>[2x]MLRSTHSPSGSSSAAPASSSSDAAMVGGGGAAAAAGSGGAPSGAKLLQILNVRVVGNGDRVVVLSHGFGTDQSAWSRVLPYLTRDHRVVLYDLVCAGSVNPEHFDFRRYDTLDSYVDDLLAILDALRIPRCAFVGHSVSAMIGILASIRRPELFAKLVLIGASPRFLNDNDYHGGFELPEIQQVFDAMAANYSAWAVGYAPLAVGADVPAAVQEFSRTLFNMRPDISLHVCRTVFNTDLRGVLGMVRSPCVVVQTTRDVSVPASVAAYLRAHLGGRTTVEFLQTEGHLPHLSAPGLLAQVLRRALARY

Strigolactones (SLs) are a class of important plant hormones mainly regulating plant architecture such as branching, which is crucial for crop yield. Different from other receptors, which could only sense hormone molecules, the receptor D14 have dual roles to sense and hydrolyze SL, demonstrating a brand-new function mode. During the hydrolysis of SL, D14 covalently binds to the D-ring at the catalytic center, then it associates with downstream protein MAX2/D3 to form D14–MAX2/D3 SCF E3 complex. This ubiquitin ligase complex will recruit the downstream transcription repressors SMXL6/7/8/D53, leading to the degradation of SMXLs/D53 through the 26S proteasome pathway.

Here, two putative SL receptors SsD14a/b and the interacting F-box protein SsMAX2 were identified in Saccharum spontaneum. The crystal structure of SsD14aΔN was determined at a resolution of 1.65 Å. SsD14a belongs to the α/β hydrolase superfamily, of which the structure consists of an α/β hydrolase core domain and a four-helix lid domain (αT1, αT2, αT3, and αT4). The catalytic triad residues of S145, D266, and H295, distributed on the loops following the β4, β6, and β7 strands, are located at the bottom of the hydrophobic substrate-binding pocket. The rest of the core domain is made up of seven β strands (β1–β7) and six α helices (α1, α2, α3, α8, α9, and α10). R310 is located at the α10 helix of SsD14a. Structure comparisons revealed that the overall structure of SsD14a was identical to those from other plants in the open state, with root-mean-square deviations (RMSD) ranging from 0.250 to 0.301 Å. Notably, the overall structure of SsD14a in the open state was apparently larger than the closed state of AtD14-CLIM (covalently linked intermediate molecule, a hydrolysis intermediate of SL molecule), thus these two structures cannot be well aligned, with an RMSD of 0.662 Å. Furthermore, results of docking approaches demonstrated extensive binding of GR24 by residues in the catalytic pocket of SsD14a. Mutagenesis analyses revealed that residue R310 at α10 helix of SsD14a was crucial for the binding with SsSMXL7/AtSMXL7 but not SsMAX2.>GPEPDMISVFIGTWNMGSVPPPKNVTSWFTSKGLGKTLDEVTVTIPHDIYVFGTQENSVGDREWLDLLRGGLKELTDLDYRPIAMQSLWNIKVAVLVKPEHENRISHVSTSSVKTGIANTLGNKGAVGVSFMFNGTSFGFVNCHLTSGNEKTARRNQNYLDILRLLSLGDRQLNADDISDRFTHLFWFGDLNYRLDMDIQEILNYISRKEFEPLLRVDQLNLEREKHKVFLRFSEEEISFPPTYRYERGSRDTYAWHKQKPTGVRTNVPSWCDRILWKSYPETHIICNSYGCTDDIVTSDHSPVFGTFEVGVTSQFISKKGLSKTSDQAYIEFESIEAIVKTASRTKFFIEFYSTCLEEYKKSFENDAQSSDNINFLKVQWSSRQLPTLKPILADIEYLQDQHLLLTVKSMDGYESYGECVVALKSMIGSTAQQF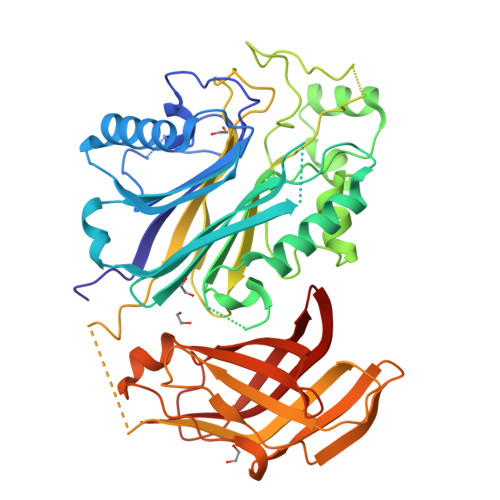LTFLSHRGEETGNIRGSMKVRVPTER[2x]>MSNRIPFPKPYTSAHDLVSLLQSRGLTIADTAKTERYLEFIGYYRLSAYMYPLLQMPKEQHRYKPNTTFDQVMMLYRFDKKLRLLIFNEIEKIEVAVRSAIVNIGSDMIGSPFWMTDGSNFIDPRKFRHTMDLIDAELGRSREDFIVHFKQTYSDAYPPAWILAEVLPFGVITNIFSNIKTARIKKSIARKFGLQVAPFESWLTIVALTRNSCCHHARVWNKQNTIRPMIPNRMTGRWIILPTDALRIYFNLCIIKYFLDIISPQNDMKAKIDALLSSYSSIDINA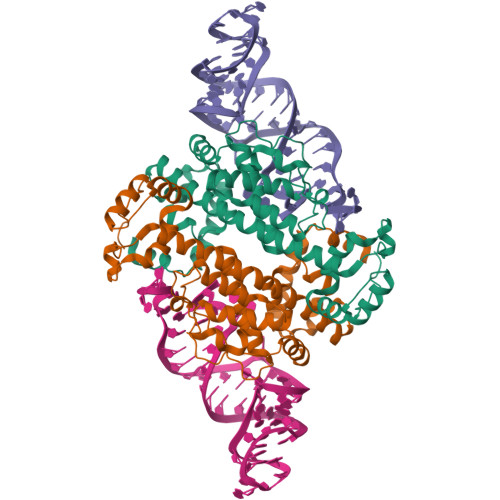MGFPRGWESEPLWQ[2x]> MLRHCTAHRRYRTAWRELLHPLPVRARKMEWLKRDAVEENEEILRRPYYTIKSY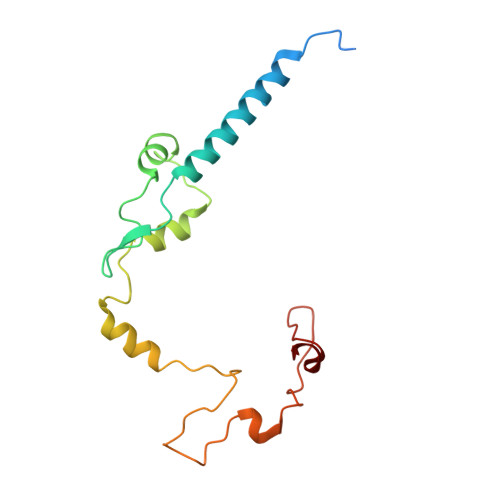ALPPAVGRQESIHNSNNIRGGMHSSHSLDLIMRQPRRVKTPEQLRALRDRLRFIGVTGPMPQATSVSTKSYTDTYGSRLRPRYPESWDTVPPHQPSRELL N~6~-methyl-N~6~-(3,4,5-trifluorophenyl)pyrido[2,3-d]pyrimidine-2,4,6-triamine | C14 H11 F3 N6 | 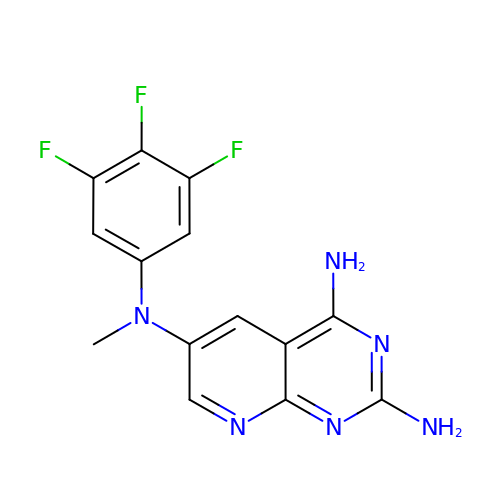RYXUPKGYPPPMSC-UHFFFAOYSA-N N~2~-(3-CARBOXYPROPANOYL)-L-ORNITHINE | C9 H16 N2 O5 | 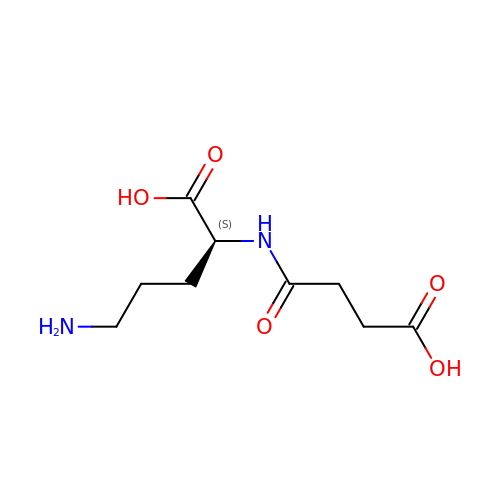VWXQFHJBQHTHMK-LURJTMIESA-N> XLET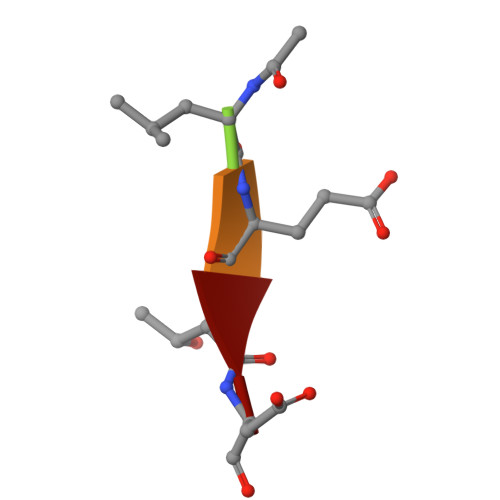D> TQFEKLMENMRNDIASHPPVEGSYAPRRGEFCIAKFVDGEWY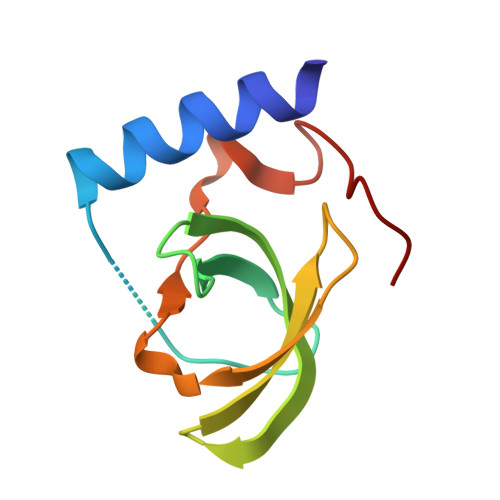RARVEKVESPAKIHVFYIDYGNREVLPSTRLGTLSPAFSTRVLPAQATE> MALKKEQHFFKGMQRDLSVSKFNPEYAFDAQNIRITAREHDTLLSVSNEKGNKEIPLQSPSGDPVVIDGVLLGQNVLNNYVTLFTKGTNDNIYRLENKGTYFETLILFSGNLNFSTDYPIESISVYENNNIQKVYWVDGLNQARVINITKDDYNNADDFDFVGTIHTSSKIEVSKVNGSGAFGQGVIQYAFTYYNKYGKETNIFRTSPLLYIAYSDRGASPEETVSCSFQINFTELDSSYDFIRVYSIHRTSIDATPTVRKVADLATDTKLYVDTGTTGEIVDPTLLLYVGGEEIAPYTMTQKDNTLFLGNYTLKRSLISTELKNQIKSDSIVTTILGGLDDAIESEWNVNTQYNSNYDLNYDSRIKGFQKGEIYRLGIQFQDNKGKWSEVVFIGDYECTERFKYTQYDTYGITLIPRFKVVISNSTTIQAIKNLGYINARGVVVFPTLEDRNILCQGILCPTVANYKDRLDNSPFVQSSWFSRPKQATETWKTEYSGTNHLSEFGEVPYFQHNEPIGSASLSEITRWEIQTSLGLVPYYNPSTTNAKDFVDGSPSEFLVDENIVTMHSPDVEFDDRLQNITNGKFKLRIIGTTHLTNTLSDISVITSTPTYGNYATGFYKGKVANMNISTSYYGGRQLSAGLFWSDNVKFQDPSPQDKLERLWMVYPWHRNGSLMNMGVPTEGTRAAALQRKIISNLKFASQNNYLPNQSVWEAEISGDANHTGITPVNSWTEGLVRIPAQANSNLGSLNYYANIDKVLTFNRSEQISEIYKNGYLIYTTKDWITDGKIADLFNNAISQTISVDQVQDWLTRIADTDKYGTEPVSMKYKSNPHLVFAFNYTESGKQLILPMKNNNNGYLAPSANSKPFWNPTAPEGAVYQDSINFTNENRAFFWLAELYRDSVVNRFGGDTEEAILNNTWLPSGDSVIIGDSINIEYTEGDTYYQRYDCLRTFAYTNEDQNSIVDIVSFMCESKVNIDGRYDKNRGQVNNLAVSPTNFNLFNPVYSQKNNFFTFRTIDYERFSINYFPNSITVTKEKSLGEDIDTWTNITLATTLDLDGDKGEIVSLNTYNNEIFCFQRRGLSNILFNSRVQIPTSDGMPIEITNGLKVSGKRYISNTIGCANKWSIAESPSGLYFIDNETNSLYLFNGEIVSLSDKLGFRQWISTHNVHVNWEPVGYNNYRSFYDKNNNDVYFTYKDHCLCYSELINQFTSFMSYEGVPAMFNVSSEFYAFKDGKMWEQFAGDYNMFFGEYKPFSITFVANAEEPNDKIFNTVEFRADSWDSDNLISNKTFDTLDVWNEYQHGTTPLTNLLGHPSPLKKKFRIWRANIPRAIANNRDRIRNTWAYIKLGMNTPNTYRTEFHDAIIHYFA;>MNVNEFSNEFDVLYNNIMSNAAPGLNEYEKSVLLTKAQEEIVKNYFEPAGNKYGKGLDDSPKRQIDFSELIKVGEGVLNTSAPTITFDKRAKVYDLPADLFLVINEAVDTNAGTKQIVPISYSDYTRLMSRPYKEPVKYQAWRIITTSINNISVELIVNSNETITDYKVRYIRRPAPIITTNLSSEYGDVTINGVSTVSECELNPIIHSEILQRAVELAKAAYQGDLQASVELGQRSE[2x]

Virus ΦcrAss001 (Kehishuvirus primarius) was the first representative of this order to be isolated in pure culture from human faecal samples. Here, we present the characterization of ΦcrAss001 using cryo-electron microscopy (cryo-EM), enabling de novo structure building and elucidation of functions for around 1,440 protein subunits constituting the virion, leading to the identification of a novel ‘crass fold’ in the distal part of the tail. The virion possesses a short non-contractile tail extending approximately 44 nm from an icosahedral capsid. The extended tail barrel formed by widely conserved paralogous ring proteins has a high capacity for storage of cargo proteins alongside the capsid cargo zone, ensuring that the proteins required for the initial stages of crassvirus infection are carried inside virions and delivered to the host cell.

At the end of the tail is a large hexameric assembly of the muzzle protein gp44. Serving as a platform for assembly of the large domain forming the distal part of the muzzle is IG2 (between residues 318–1021). This domain is formed by insertions into loops between IG2 strands E–F (residues 453–904) and G–H (residues 940–1012), with the E–F insertion making up the bulk of this region. As this domain adopts a fold with no significant structural similarity to known protein domains, we refer to it here as the ‘crass fold’. The muzzle is gated by a loop within blade 4 of the propeller. One role of the muzzle is likely to be the formation of this constriction, preventing leakage of DNA and proteins contained in the capsid and tail until infection is initiated. Owing to the restricted channel diameter above and below the gate, and interactions at the inter-subunit interfaces, opening it would require conformational rearrangements of the IG and crass domains. The crass domain, owing to its location on the tail tip and the presence of multiple exposed surface loops, is likely to have a role in contacting the cell surface, thus initiating these conformational changes. A further region of density inside the tail was observed at its distal end, next to the ring-joining domain of the muzzle protein. This region corresponds to 6 copies of a 14-residue segment containing an α-helix.> AAPNDPSYRQQWHYFGNYGVKANKVWDRGFTGQGVVVSVVDTGILDHVDLNGNMLPGYDFISSAPNARDGDQRDNNPADEGDWFDNWDCGGYPDPRREKKFSTWHGSHVAGTIAAVTNNGVGVAGVAYGAKVIPVRVLGKCGGYDSDITDGMYWSAGGHIDGVPDNQNPAQVVNMSLGGGGGCSQNSQRMIDKTTNLGALIVIAAGNENQDASRTWPSSCNNVLSVGATTPKGKRAPFSNYGARVHLAAPGTNILSTIDVGQAGPVRSSYGMKAGTSMAAPHVSGVAALVISAANSIGKTLTPSELSDILVRTTSRFNGRLDRGL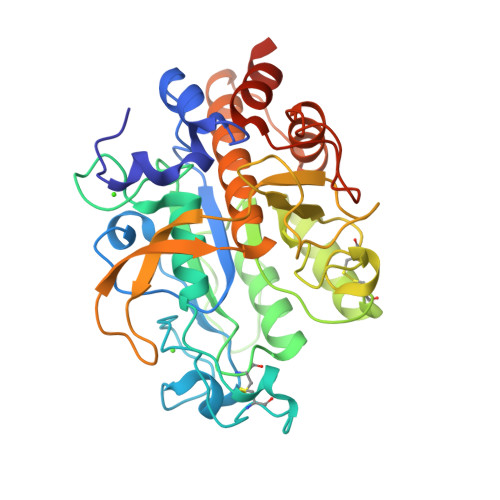GSGIVDANAAVNAVLGDQNLEHHHHHH The core kinase cascade is modulated by adaptor proteins, SAV1 (Salvador, also known as WW45) and MOB1 (encoded by MOB1A and MOB1B in human), both of which work to promote Hippo pathway signaling. MOB1 directly binds to LATS1 and LATS2, and additionally to two related kinases, NDR1, (gene name STK38) and NDR2 (gene name STK38L) via a specialized MOB1-binding domain N-terminal to the kinase domain (15; also see accompanying manuscript by Xiong et al., 2017). Key to its function as a Hippo pathway activator is the ability of MOB1 to bind directly to MST1 and MST2 kinases. We demonstrate that autophosphorylation of MST1 and MST2 on several threonine residues provides multiple MOB1 binding sites with varying binding affinities which in turn contribute to a redundancy of MST1-MOB1 protein interactions in cells.

Peptide overlay analysis (here referred to as Far-Western) revealed that peptides bearing phosphorylated forms of T353 and T367 consistently gave the highest binding signals across the array; nonphosphorylated versions of these peptides generated little to no binding signal. MST1 T353 and T367 peptides displayed high phospho-dependent binding affinities for MOB1A, with Kds of 280 nm and 680 nm for the phosphorylated peptides, respectively, and no detectable binding for the nonphosphorylated peptides. The observed binding modes revealed by these structures are in close agreement with the binding modes reported previously for a yeast Nud1 derived phosphopeptide in complex with human MOB1A, as well as a MST2 T378 phosphopeptide in complex with human MOB1B (see ref 21, 22). As predicted by prior mutational data, the MST1 pT353 and pT367 phosphopeptides bound to the MOB1A phospho-binding pocket first identified by Rock et al., with the phosphate of the P0 threonine directly coordinated by K153, R154 and R157. The p + 1 side chains of M354 and M368 on MST1-pT353 and MST1-pT367 peptides respectively resided in an expansive hydrophobic surface composed by A89, A92, Y93, Y95, F156 and A160 side chains on MOB1A. The p + 2 side chains of I355 and V369 in MST1-pT353 and MST1-pT367 peptides respectively pointed to a distinct surface composed by M87, Y95 and the aliphatic portion of the E94 side chain on MOB1A. Thus, the hydrophobic nature of the p + 1 to p + 3 binding surfaces explained the consensus preferences for hydrophobic residues at these positions. Ni et al. recently reported the crystal structure of MOB1 bound to an extended phosphopeptide derived from MST2 encompassing T378 (ref 21). This considerably longer peptide sequence (31 residues versus the 15-residue peptides described here) appeared suboptimal in having disfavored basic residues at positions p + 2 and p + 3, and yet was reported to bind more tightly (120 nm) to MOB1B than did the consensus matching shorter MST1 pT353 peptide.

> MSFLFSSRSSKTFKPKKNIPEGSHQYELLKHAEATLGSGNLRQAVMLPEGEDLNEWIAVNTVDFFNQINMLYGTITEFCTEASCPVMSAGPRYEYHWADGTNIKKPIKCSAPKYIDYLMTWVQDQLDDETLFPSKIGVPFPKNFMSVAKTILKRLFRVYAHIYHQHFDSVMQLQEEAHLNTSFKHFIFFVQEFNLIDRRELAPLQELIEKLGSKDR;> VASTMTDGANTMIEP> MKHDYTNPPWNAKVPVQRAMQWMPISQ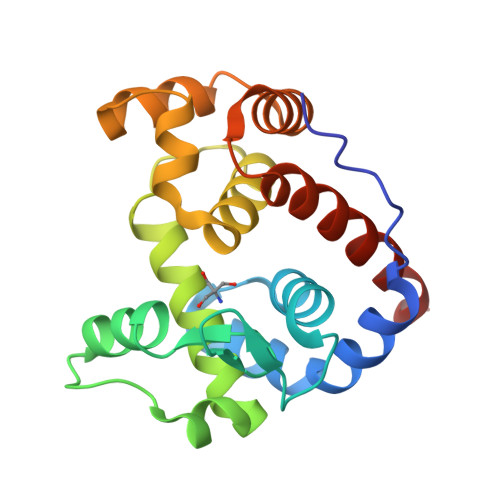KAGAAWGVDPQLITAIIAIESGGNPNAVSKANAIGLMQLKASTSGRDVYRRMGWSGEPTTSELKNPERNISMGAAYLNILETGPLAGIEDPKVLQYALVVSYANGAGALLRTFSSDRKKAISKINDLDADEFLEHVARNHPAPQAPRYIYKLEQALDAMLEHHHHHH> MLPSQSPAIFTVSRLNQTVRLLLEHEMGQVWISGEISNFTQPASGHWYFTLKDDTAQVRCAMFRNSNRRVTFRPQHGQQVLVRANITLYEPRGDYQIIVESMQPAGEGLLQQKY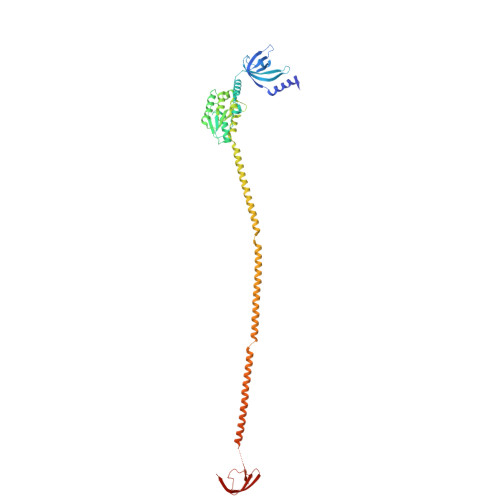EQLKAKLQAEGLFDQQYKKPLPSPAHCVGVITSKTGAALHDILHVLKRRDPSLPVIIYPAAVQGDDAPGQIVRAIELANQRNECDVLIVGRGGGSLEDLWSFNDERVARAIFTSRIPVVSAVGAETDVTIADFVADLRAPTPSAAAEVVSRNQQELLRQVQSTRQRLEMAMDYYLANRTRRFTQIHHRLQQQHPQLRLARQQTMLERLQKRMSFALENQLKRTGQQQQRLTQRLNQQNPQPKIHRAQTRIQQLEYRLAETLRAQLSATRERFGNAVTHLEAVSPLSTLARGYSVTTATDGNVLKKVKQVKAGEMLTTRLEDGWIESEVKNIQPVKKSRKKVH1-[(2S)-4-(5-phenyl-1H-pyrazolo[3,4-b]pyridin-4-yl)morpholin-2-yl]methanamine 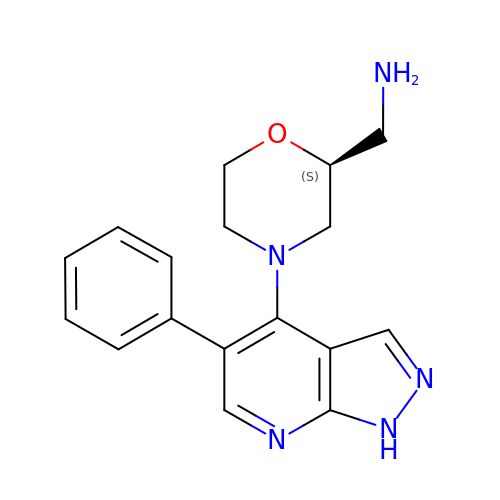| C17 H19 N5 O | YBRZCAKSBYWZTC-ZDUSSCGKSA-N>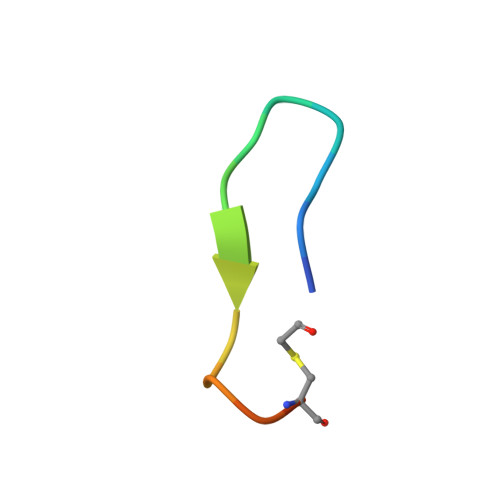 FWDSWGYWYGPWDCGKX>[2x]CCAGGCTGCAA

The G-quadruplex and the i-motif are two noncanonical structures that have been studied extensively, and each is characterized by specific types of noncanonical interactions. G-quadruplexes (G4s) are formed from G-rich sequences and contain stacked guanosine tetrads, organized in a cyclic hydrogen bonding arrangement between the Hoogsteen and Watson–Crick faces of neighboring nucleobases. The DNA i-motif is characterized by the formation of hemiprotonated C–C+ parallel-stranded base pairs, which are organized to allow two duplexes to intercalate in an antiparallel fashion to form a quadruplex structure. As part of a screen to probe the structural diversity of DNA, we have crystallized many short DNA oligonucleotides, including d(CCAGGCTGCAA).

Here, we describe the crystal structure of the DNA oligonucleotide, d(CCAGGCTGCAA), that self-associates to form a quadruplex structure containing two central antiparallel G-tetrads and six i-motif C–C+ base pairs. The asymmetric unit contains two oligonucleotides (Chains A and B) that interact as a dimer. Two dimers interact through crystal symmetry (symmetry molecules designated as Chains A' and B') to form a tetramer. This tetramer contains a number of distinct structural motifs, including a central G-quadruplex, a base triple interaction, a structurally variable spacer region, and a terminal i-motif. The central G-quadruplex is composed of two symmetrically equivalent G-tetrads, each of which is formed through two G4 and two G5 residues. The eight guanosines coordinate directly with a central cation that is located between the two G-tetrad planes. Both the native and U7-Br oligonucleotides were crystallized in the presence of barium chloride, and a strong (11 σ) anomalous difference electron density peak between the two G-tetrads was observed in both native and derivative structures. Flanking each side of the G-quadruplex is an A–A–T base triple. The d(CCAGGCTGCAA) tetramer is capped at either end by i-motifs. The i-motif is comprised of three C–C+ base pairs between C1, C2, and C9 residues of the dimers.>[2x]APITAYSQQTRGLLGCIITSLTGRDKNQVEGEVQVVSTATQSFLATCVNGVCWTVYHGAGSKTLAGPKGPITQMYTNVDQDLVGWQAPPGARSLTPCTCGSSD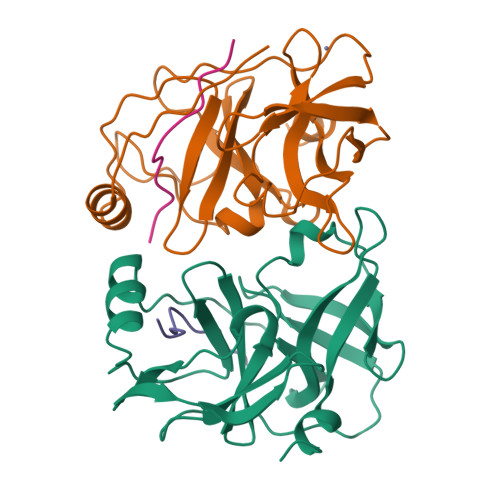LYLVTRHADVIPVRRRGDSRGSLLSPRPVSYLKGSSGGPLLCPSGHAVGIFRAAVCTRGVAKAVDFVPVESMETTMRASKKKK;>[2x]KGSVVIVGRIILSGRK> MVKIVYPNAKDFFSFINSITNVTDSIILNFTEDGIFSRHLTEDKVLMAIMRIPKDVLSEYSIDSPTSVKLDVSSV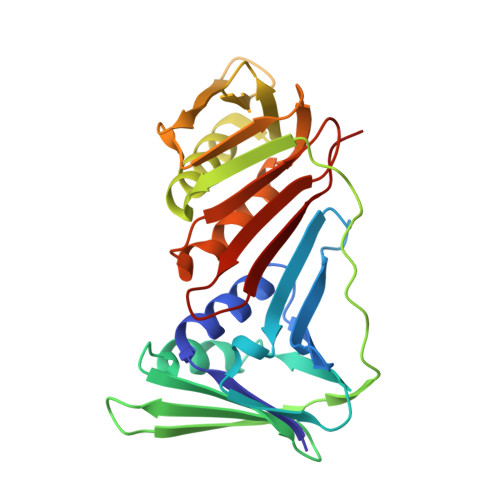KKILSKASSKKATIELTETDSGLKIIIRDEKSGAKSTIYIKAEKGQVEQLTEPKVNLAVNFTTDESVLNVIAADVTLVGEEMRISTEEDKIKIEAGEEGKRYVAFLMKDKPLKELSIDTSASSSYSAEMFKDAVKGLRGFSAPTMVSFGENLPMKIDVEAVSGGHMIFWIAPRL>GIKVFLHERELWLKFHEVGTEMIITKAGRRMFPSYKVKVTGLNPKTKYILLMDIVPADDHRYKFADNKWSVTGKAEPAMPGRLYVHPDSPATGAHWMRQLVSFQKLKLTNNHLDPFGHIILNSMHKYQPRLHIVKADEN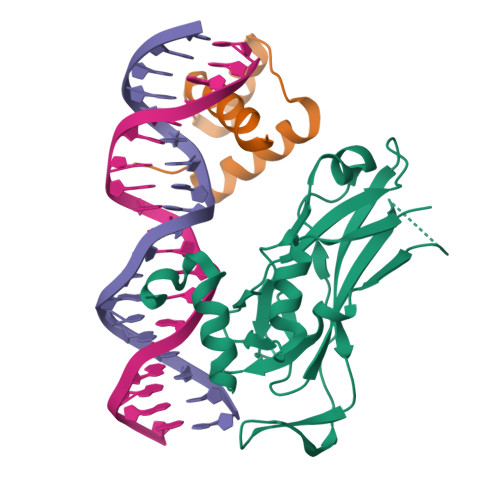NGFGSKNTAFCTHVFPETAFIAVTSYQNHKITQLKIENNPFAKGFRG[2x];>RVLFSQAQVYELERRFKQQRYLSAPERDQLASVLKLTSTQVKIWFQNRRYKSK[2x]>[2x]DDAAIQQTLAKMGIKSSDIQPAPVAGMKTVLTNSGVLYITDDGKHIIQGPMYDVSGTAPVNVTNKMLLK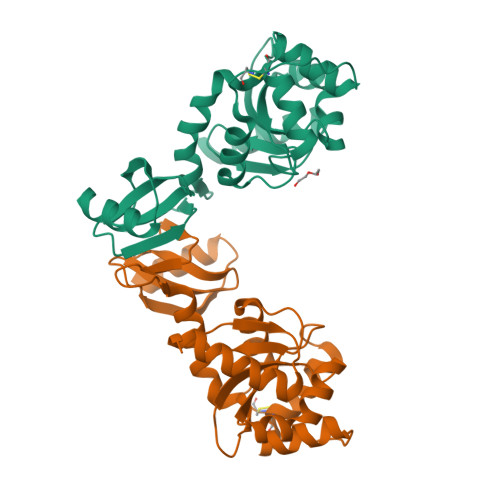QLNALEKEMIVYKAPQEKHVITVFTDITCGYSHKLHEQMADYNALGITVRYLAFPRQGLDSDAEKEMKAIWCAKDKNKAFDDVMAGKSVAPASCDVDIADHYALGVQLGVSGTPAVVLSNGTLVPGYQPPKEMKEFLDEHQKMTSGK> MGHHHHHHMPVGVFSRQILKNVPHLEVFLEDSVVYKPKGPEGLSAVAGWGYKSTARKAMQKAREWRLPYLALEDGFLRSVGLGHEAPPLSLIVDPVGIYYDATRPSLLENLLNFGGWETPELMDQAERALKLIRDHKISKYNRGKPVPRGYFTPYRERVLLIDQTYGDMSVRLGLADEDTFREMYFAALEENPGAEIYVKVHPEVIVGRKKGYLARMKLHRSVKVIREEFNPVDLLSHFDRIYTVSSQMGFEGLMLGKEVICFGMPFYAGWGLTRDGKRCERRKRRRTLLELFAAA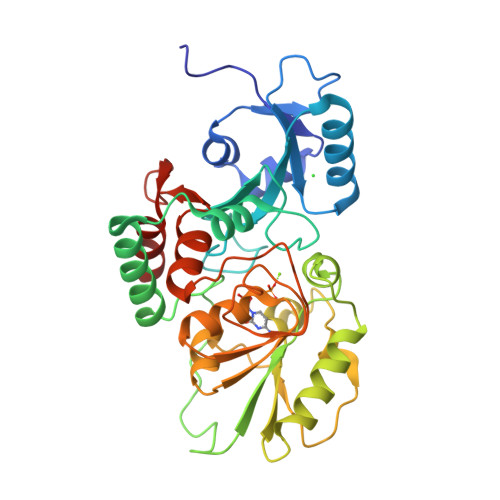YLLYPRYINPATGKPGNIFDVINHLIGGKG>[4x]MKIVLAYSGGLDTSIILKWLKETYRAEVIAFTADIGQGEEVEEAREKALRTGASKAIALDLKEEFVRDFVFPMMRAGAVYEGYYLLGTSIARPLIAKHLVRIAEEEGAEAIAHGATGKGNDQVRFELTAYALKPDIKVIAPWREWSFQGRKEMIAYAEAHGIPVPVTQEKPYSMDANLLHISYEGGVLEDPWAEPPKGMFRMTQDPEEAPDAPEYVEVEFFEGDPVAVN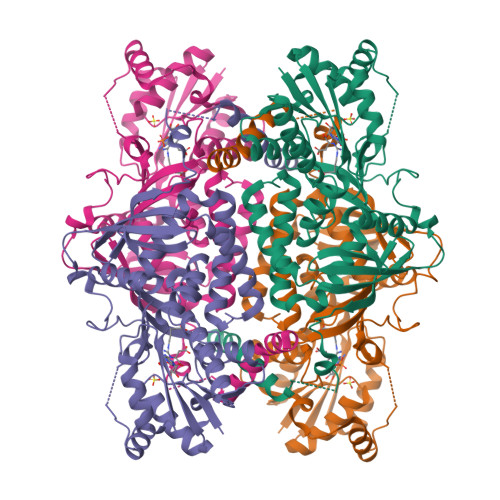GERLSPAALLQRLNEIGGRHGVGRVDIVENRFVGMKSRGVYETPGGTILYHARRAVESLTLDREVLHQRDMLSPKYAELVYYGFWYAPEREALQAYFDHVARSVTGVARLKLYKGNVYVVGRKAPKSLYRQDLVSFDEAGGYDQKDAEGFIKIQALRLRVRALVEREGHGA6-(6,7-dihydro-4H-thieno[3,2-c]pyridin-5-yl)pyridin-3-amine | C12 H13 N3 S 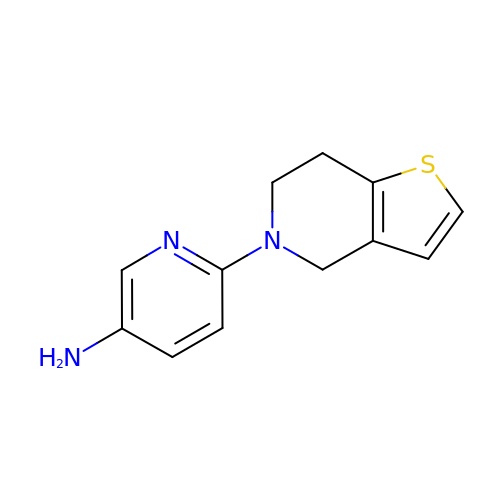| VEJCYGREDNZFMG-UHFFFAOYSA-N> MKFFYSDQNVDSRDPVQLNLLYVQARDDILNGSHPVSFDKACEFAGYQCQIQFGPHNEQKHKPGFLELKDFLPKEYIKQKGERKIFMAHKNCGNMSEIEAKVRYVKLARSLKTYGVSFFLVKEKMKGKNKLVPRLLGITKECVMRVDEKTKEVIQEWSLTNIKRWAASPKSFTLDFG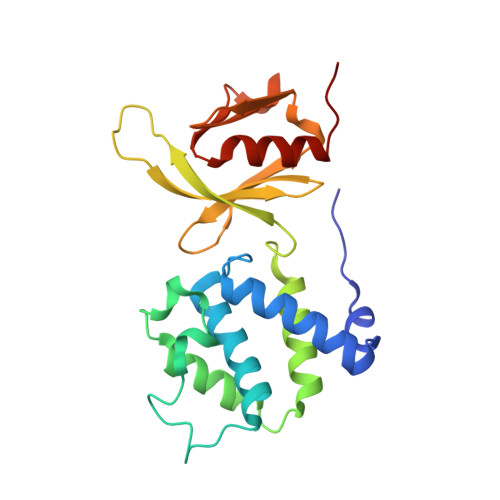DYQDGYYSVQTTEGEQIAQLIAGYIDIIL N-{6-[4-(ethenylsulfonyl)-1,4-diazepan-1-yl]-2-(pyridin-2-yl)pyrimidin-4-yl}-beta-alanine | C19 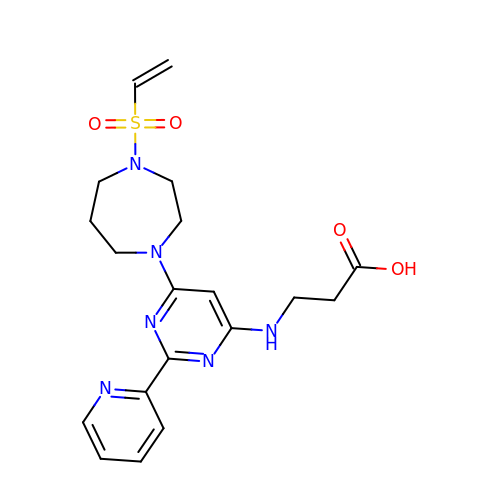H24 N6 O4 S | CPNWZGJHUIZVEZ-UHFFFAOYSA-N>STNDNIKDLLDWYSSGSDTFTNSEVLDNSLGSMRIKNTDGSISLIIFPSPYYSPAFTKGEKVDLNTKRTKKSQHTSEGTYIHFQISGVTNTEKLPTPIELPLKVKVHGKDSPLKYWPKFDKKQLAISTLDFEIRHQLTKIHGLYRSSDKTGGYWKITMNDGSTYQSDLSKKFEYNTEKPPINIDEI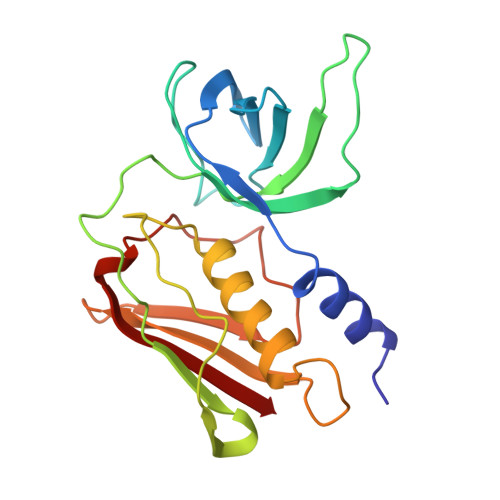KTIEAEIN[2x]> GAMGQKAQQKNGYQEIRVEVMGGYTPELIVLKKSVPARIVFDRKDPSPCLDQIVFPDFGVHANLPMGEEYVVEITPEQAGEFSFACGMNMMHGK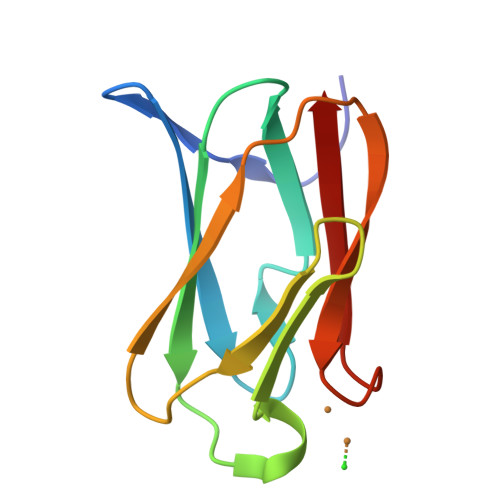MIVE>GPDSMASLQRKGLQARILTSEEEEKLKRDQTLVSDFKQQKLEQEAQKNWDLFYKRNSTNFFKDRHWTTREFEELRSCREFEDQKLTMLEAGCGVGNCLFPLLEEDPNIFAYACDFSPRAIEYVKQNPLYDTERCKVFQCDLTKDDLLDHVPPESVDVVMLIFVLSAVHPDKMHLVLQNIYKVLKPGKSVLFRDYGLYDHAMLRFKASSKLGENFYVRQDGTRSYFFTDDFLAQLFMDTGYEEVVNEYVFRETVNKKEGLCVPRVFLQSKFLKPPK[2x]

Methylation of cytosine 32 in the anticodon loop of tRNAs to 3-methylcytosine (m3C) is crucial for cellular translation fidelity. Here, we report the cryo-electron microscopy structure of the human m3C tRNA methyltransferase METTL6 in complex with seryl-tRNA synthetase (SerRS) and their common substrate tRNASer. We show that SerRS acts as the tRNASer substrate selection factor for METTL6. We demonstrate that SerRS augments the methylation activity of METTL6 and that direct contacts between METTL6 and SerRS are necessary for efficient tRNASer methylation.

Despite attempts to crystallize the complex, we could only achieve two crystal forms of METTL6 bound to SAH and the complex disintegrated during cryo-EM grid preparation. To determine whether tRNA binding to METTL6 induces conformational changes in the enzyme, we compared our structural model to the crystal structures of METTL6 bound to either SAM or SAH, but without an RNA ligand. The methyltransferase core of all models aligns well. Deviations occur exclusively in the m3C-RBD, in particular in the divergent N-terminal region, the substrate-binding loop and the β-extension. All RNA-free structures display disordered substrate-binding loops, which seem to adopt their shape only in contact with the tRNA, and a conserved helix following the substrate-binding loop is rearranged on interaction with the ligand. Our data suggest some degree of flexibility in the region of the β-extension hairpin, a region that is completely unresolved in the crystal structures, suggesting its plasticity for tRNASer accommodation. Thus, while the core of METTL6 is rigid, parts of the m3C-RBD seem to be more ductile, to accommodate the tRNA.>[4x]MTREELLRENIELAKEHIEIMREILELLQKMEELLEKARGADED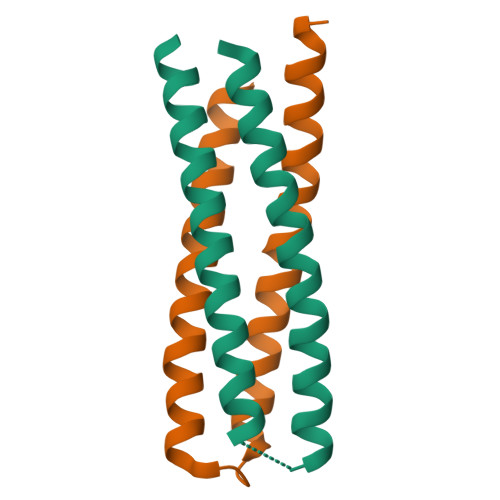VAKTIKELLRRLKEIIERNQRIAKEHEYIARERS;>[4x]GTERKLLERSRRLQEESKRLLDEMAEIMRRIKKLLKKARGADEKVLDELRKIIERIRELLDRSRKIHERSEEIAYKEE> KLAFRHHRYDDLVRTLYKVQNECPGITRVYSIGRSVEGRHLYVLEFS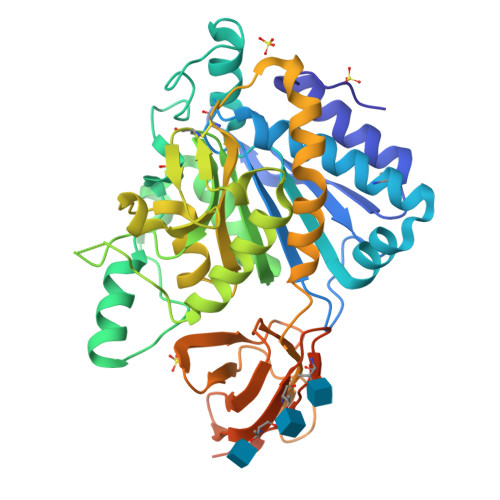DHPGIHEPLEPEVKYVGNMHGNEALGRELMLQLSEFLCEEFRNRNQRIVQLIQDTRIHILPSMNPDGYEVAAAQGPNKPGYLVGRNNANGVDLNRNFPDLNTYIYYNEKYGGPNHHLPLPDNWKSQVEPETRAVIRWMHSFNFVLSANLHGGAVVANYPYDKSFEHRVRGVRRTASTPTPDDKLFQKLAKVYSYAHGWMFQGWNCGDYFPDGITNGASWYSLSKGMQDFNYLHTNCFEITLELSCDKFPPEEELQREWLGNKEALIQFLEQVHQGIKGMVLDQNYNNLANAVISVSGINHDVTSGDHGDYFRLLLPGIYTVSATAPGYDPETVTVTVGPAEPTLVNFHLKRSIPQVSPVRRAPSRRHGVRAKVQPQARKKEMEMRQLQRGPA> GCSQHLVEVGKGYSCTSVNTTVFRNNSLVTHGDEQYISYYDNDGYLVLGKRKLDSEQWTLHRTQYQGNVKDAHNIISMMIDGEGYIHVSFDHHGHPLNYCRSIAPGSLELGDKMPMTGVDEGNVTYPEFYPLSGGDLLFVYRSGSSGRGNLVMNRYSLKEHKWTRVQDILIDGENKRNAYWQLYVDEKGTIHLSWVWRETWHVETNHDICYARSFDNGVTWYKTSGERYELPIKLSNAEYACRLPQNCELINQTSMSADAGGNPYIATYWREPNSDVPQYRIVWNDGKMWHQRQITDRQTPFTLKGG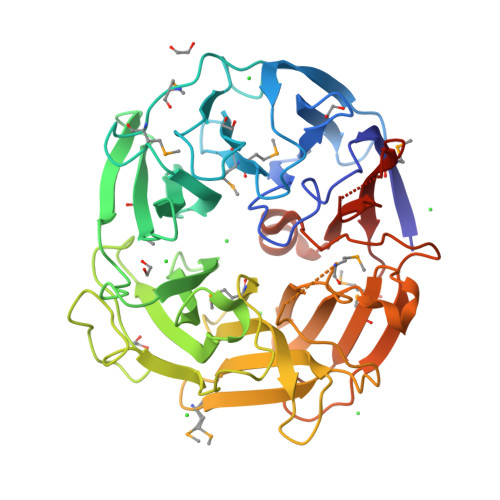GTKMIPIARPRIVVEGGEVFYIFRDEERGSRVSMAHATDVGTSKWTITDLTDFSVDAWEPSHDTELWKKQRKLHLFVQHTRQGDGERTAEIEPQMIYVLETNMDTNK>[2x]TRKAVIGYYFIPTNQINNYTETDTSVVPFPVSNITPAKAKQLTHINFSFLDINSNLECAWDPATNDAKARDVVNRLTALKAHNPSLRIMFSIGGWYYSNDLGVS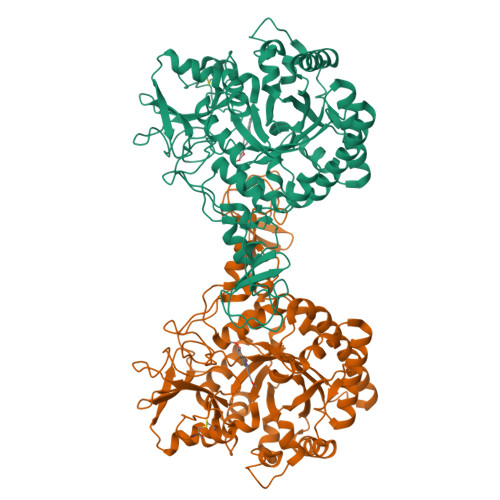HANYVNAVKTPASRAKFAQSCVRIMKDYGFDGVDIDWEYPQAAEVDGFIAALQEIRTLLNQQTITDGRQALPYQLTIAGAGGAFFLSRYYSKLAQIVAPLDYINLMTYDLAGPWEKVTNHQAALFGDAAGPTFYNALREANLGWSWEELTRAFPSPFSLTVDAAVQQHLMMEGVPSAKIVMGVPFYGRAFKGVSGGNGGQYSSHSTPGEDPYPSTDYWLVGCEECVRDKDPRIASYRQLEQMLQGNYGYQRLWNDKTKTPYLYHAQNGLFVTYDDAESFKYKAKYIKQQQLGGVMFWHLGQDNRNGDLLAALDRYFNAADYDDSQLDMGTGLRYTGVGPGNLPIMTAPAYVPGTTYAQGALVSYQGYVWQTKWGYITSAPGSDSAWLKVGRV> ATPVPKQFKAVKPVGDRVLVKVDKEEAKSVGGVLLPASVRNKPTAGSIIALGDAKSVKLSDKVIYSKFAGTELELGGAEHVLLKEEDVIGVLSASEKIAQLKPLSDRILIKGAKAEDKTSGGVLLATESAEKPTFGTVVAVGEGREDEETKALVKPNVTVGATVMYS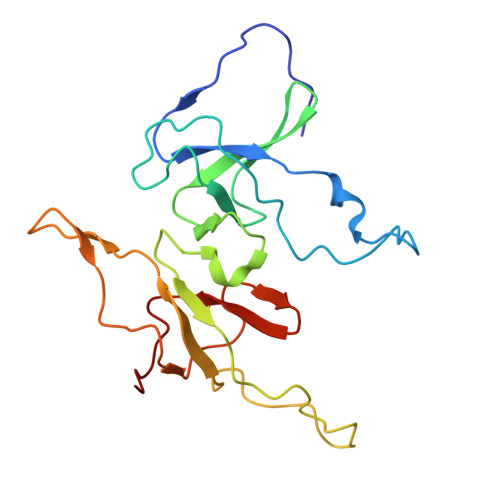KYSGTEFEEDGDNYIVVRESDILAQLS> GAGCAGACGTG;> ACCGCACTCA;> CAGGT;> TCTGAGTGCC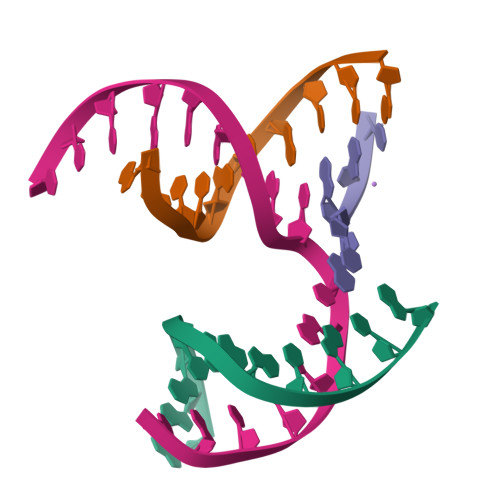GTCTGC>[6x]MADVFHLGLTKAMLDGATLAIVPGDPERVKRIAELMDNATFLASHRE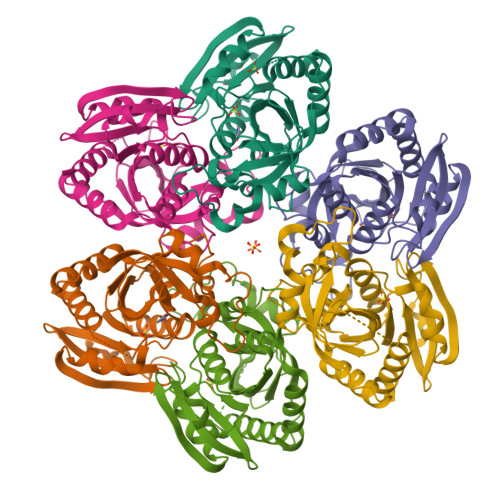YTSYLAYADGKPVVICSTGIGGPSTSIAVEELAQLGVNTFLRVGTTGAIQPHVNVGDVIVTQASVRLDGASLHFAPMEFPAVANFECTTAMVAACRDAGVEPHIGVTASSDTFYPGQERYDTVTGRVTRRFAGSMKEWQDMGVLNYEMESATLFTMCATQGWRAASVAGVIVNRTQQEIPDEATMKKTEVSAVSIVVAAAKKLLA>CPRFLKVKNWETEVVLTDTLHLKSTLETGCTEYICMGSIMHPSQHARRPEDVATKDQLFPLAKEFIDQYYSSIKRFGSKAHMERLEEVNKEIDTTSTYQLKDTELIYGAKHAWRNASRCVGRIQWSKLQVFDARDCTTAHGMFNYICNHVKYATNKGNLRSAITIFPQRTDGKHDFRVWNSQLIRYAGYKQPDGSTLGDPANVQFTEICIQQGWKPPRGRFDVLPLLLQANGNDPELFQIPPELVLEVPIRHPKFEWFKDLGLKWYGLPAVSNMLLEIGGLEFSACPFSGWYMGTEIGVRDYCDNSRYNILEEVAKKMNLDMRKTS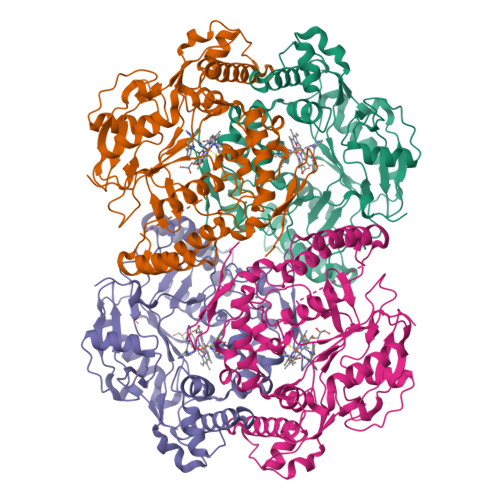SLWKDQALVEINIAVLYSFQSDKVTIVDHHSATESFIKHMENEYRCRGGCPADWVWIVPPMSGSITPVFHQEMLNYRLTPSFEYQPDPWNTHVW[4x]>[8x]DSS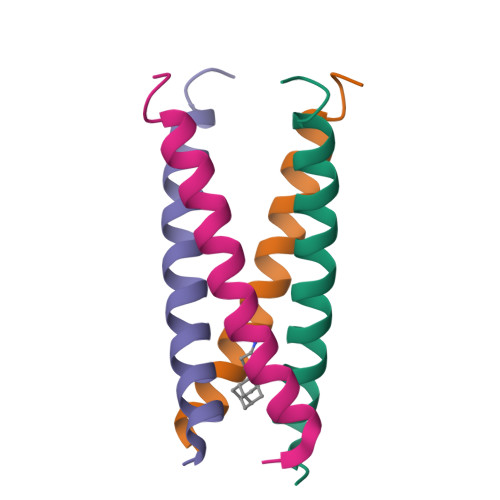DPLAVAASIIGILHLILWILDRLFFKSIYRFFEHGLKR> MLAGVKKDIEKLYEAVPQLSNVFKIEDKIGEGTFSSVYLATAQLQVGPEEKIALKHLIPTSHPIRIAAELQCLTVAGGQDNVMGVKYCFRKNDHVVIAMPYLEHESFLDILNSLSFQEVREYMLNLFKALKRIHQFGIVHRDVKPSNFLYNRRLKKYALVDFGLAQGTHDTKIELLKFVQSEAQQERCSQNKPASLTCDCYATDKVCSICLSRRQQVAPRAGTPGFRAPEVLTKCPNQTTAIDMWSAGVIFLSLLSGRYPFYKASDDLTALAQIMTIRGSRETIQAAKTFGKSILCSKEVPAQDLRKLCERLRGAGAGGWNEVPDEAYDLLDKLLDLNPASRITAEEALLHPFFKDMSL;> GPGTRTGRLKKPFVKVEDMSQLYRPFYLQLTNMPFINYSIQKPCSPFDVDKPSSMQKQTQVKLRIQTDGDKYGGTSIQLQLKEKKKKGYCECCLQKYEDLETHLLSEQHRNFAQSNQYQVVDDIVSKLVFDFVEYEKDTPKKKR

CDC7 is an essential Ser/Thr kinase that acts upon the replicative helicase throughout the S phase of the cell cycle and is activated by DBF4. CDC7 possesses the canonical bilobal kinase fold, which is interrupted by unique kinase inserts (KIs). The structures reveal a zinc-finger domain at the end of the kinase insert 2 that pins the CDC7 activation loop to motif M of DBF4 and the C lobe of CDC7. We conclude that CDC7 activity is controlled by DBF4 at two levels: (1) via ordering of the activation loop dependent on the ZF domain-DBF4 motif M interactions; and (2) via the control of αC insertion through by DBF4 motif C (Hughes et al., 2012).

Crystals were obtained with CDC7(Δ1–36/Δ228–345/Δ467–533)-DBF4MC heterodimer, which retained full activity compared with the matched control harboring complete KI-2 and KI-3. To facilitate crystallization of the catalytically competent constructs, we replaced 22 KI-3 residues retained in the previously characterized construct, but not visible in the structure, with a pentapeptide linker Gly-Ala-Gly-Ala-Gly (the deletion designated Δ467–533). X-ray diffraction data were collected using crystals grown in the presence of the ATP-competitive CDC7 inhibitor XL413 (Koltun et al., 2012). Crystal structures of the XL413-bound and nucleotide-bound complexes were refined to 1.4 and 1.8 Å resolution, respectively. The structures are highly similar to that of the previously characterized construct (Hughes et al., 2012), with the root-mean-square deviations (RMSDs) of common αC atom positions between the two constructs of ∼0.6 Å. Here, residues Cys351, Cys353, Cys360, and Cys363, all which are invariant among metazoan CDC7 orthologs, coordinate a single metal ion, nucleating zinc-finger (ZF) domain. We confirmed the presence of a Zn atom in the structure by anomalous diffraction. The ZF domain nestles on motif M of DBF4, sandwiching it against the C lobe of CDC7. Crucially, this interaction pins back the beginning of the CDC7 activation loop, inducing it to adopt a stable conformation. The current structures will be informative for the design of competitive active-site antagonists of CDC7 kinase.N-SUCCINYL METHIONINE | C9 H15 N O5 S | 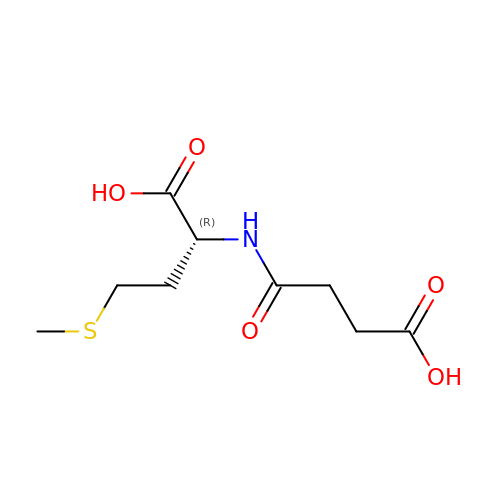CZFFMUMOBDIXJU-ZCFIWIBFSA-N2,6-dichloro-N-(difluoromethyl)-4-[3-(piperidin-4-yl)propyl]-N-(1,3,5-trimethyl-1H-pyrazol-4-yl)benzenesulfonamide 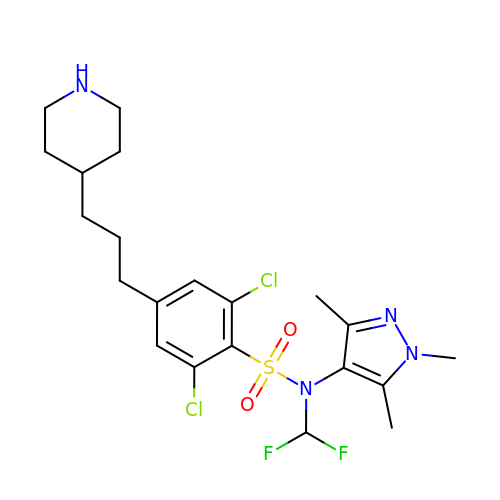| C21 H28 Cl2 F2 N4 O2 S | WZELAXINRXHZED-UHFFFAOYSA-N1-phenyl-3-(1,2,3-thiadiazol-5-yl)urea | C9 H8 N4 O S | 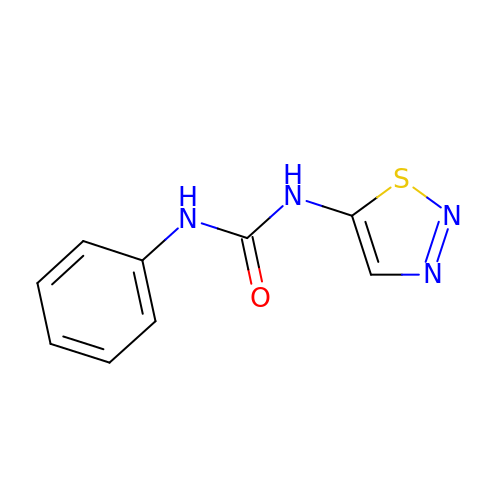HFCYZXMHUIHAQI-UHFFFAOYSA-N>[2x]MSLDGIDDLEFVDENYYISPSLDTLATL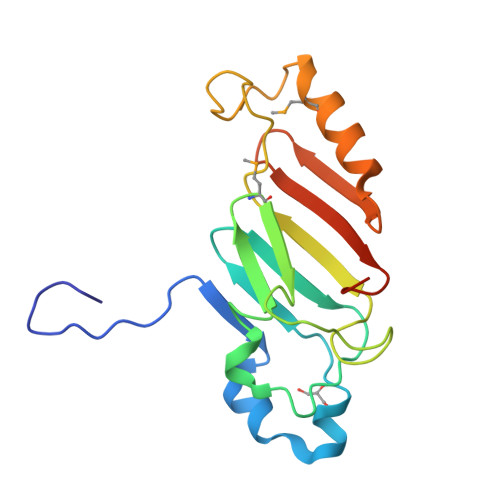SKYEIQKVENLVVGNKQYGKIEFLDPVDLSDIPLGSICDDLVVFQPMSVLLYNNSTNVPEKGKGLNVRARISCYNCYPLDKSTRKPIKDPNHRIMERYSEKLKKIPHTHFESYDPASGTYCFTVDHALEGHHHHHH> MKA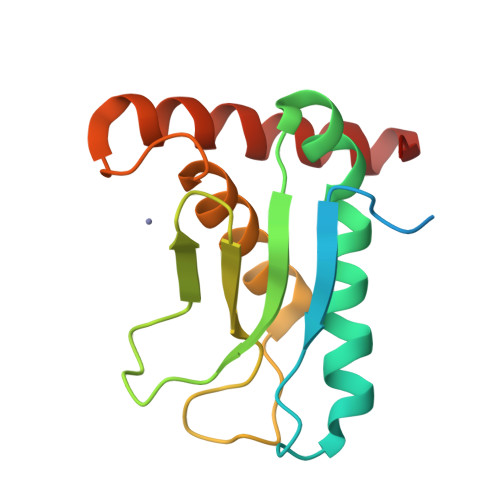EGIKSPSAKYHDMAGSQRIPHKNPHIQKVAVLQSKPNKEDALNLIKEIAHKVSYLMKENHFKVTNLVEFYPRDQRLLGMNVNHGSKIMLRLRCSTDEFQFLPMECIMGTMLHQLTHNLFGPHDKKFYNKLDELIGRQWVIEQRGLY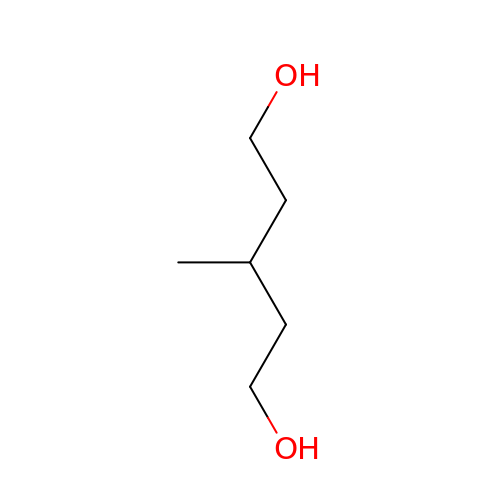3-methylpentane-1,5-diol | C6 H14 O2 | SXFJDZNJHVPHPH-UHFFFAOYSA-N> TDTTLPPDDSLDRIEPVDIEQEMQRSYIDYAMSVIVGRALPEVRDGLKPVHRRVLYAMFDSGFRPDRSHAKSARSVAETMGNYHPHGDASIYDSLVRMAQPWSLRYPLVDGQGNFGSPGNDPPAAMRYTEARLTPLAMEMLREIDEETVDFIPNYDGRVQEPTVLPSRFPNLLANGSGGIAVGMATNIPPHNLRELADAVFWALENHDADEEETLAAVMGRVKGPDFPTAGLIVGSQGTADAYKTGRGSIRMRGVVEVEEDSRGRTSLVITELPYQVNHDNFITSIAEQVRDGKL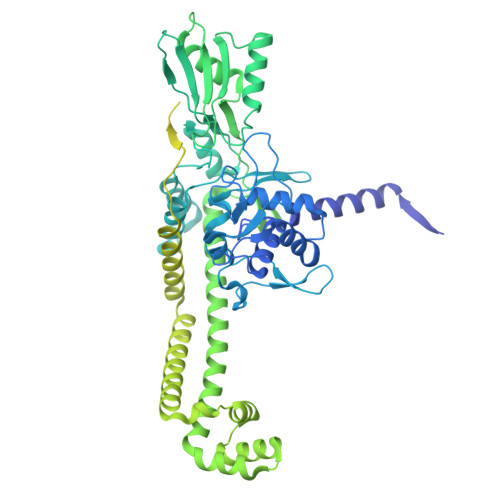AGISNIEDQSSDRVGLRIVIEIKRDAVAKVVINNLYKHTQLQTSFGANMLAIVDGVPRTLRLDQLIRYYVDHQLDVIVRRTTYRLRKANERAHILRGLVKALDALDEVIALIRASETVDIARAGLIELLDIDEIQAQAILDMQLRRLAALERQRIIDDLAKIEAEIADLEDILAKPERQRGIVRDELAEIVDRHGDDRRTRIIAIDGDVSDEDLIAREDVVVTITETGYAKRTKTDLYRSQKRGGKGVQGAGLKQDDIVAHFFVCSTHDLILFFTTQGRVYRAKAYDLPEASRTARGQHVANLLAFQPEERIAQVIQIRGYTDAPYLVLATRNGLVKKSKLTDFDSNRSGGIVAVNLRDNDELVGAVLCSAGDDLLLVSANGQSIRFSATDEALRPMGRATSGVQGMRFNIDDRLLSLNVVREGTYLLVATSGGYAKRTAIEEYPVQGRGGKGVLTVMYDRRRGRLVGALIVDDDSELYAVTSGGGVIRTAARQVRKAGRQTKGVRLMNLGEGDTLLAIARNAEESGDDNAVDANGADQTGN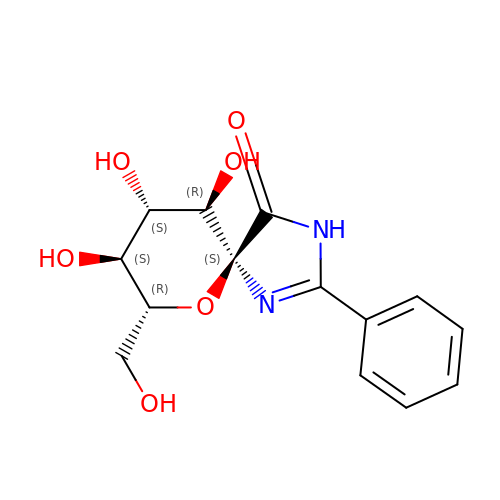(5~{S},7~{R},8~{S},9~{S},10~{R})-7-(hydroxymethyl)-8,9,10-tris(oxidanyl)-2-phenyl-6-oxa-1,3-diazaspiro[4.5]dec-1-en-4-one | C14 H16 N2 O6 | BCSCGCOVRJYILO-QEGBUVANSA-N>MNRQELITEALKARDMAYAPYSKFQVGAALLTKDGKVYRGCNIENAAYSMCNHAEQTALFKAVSEGDTEFQMLAVAADTPGPVSPCGACRQVISELCTKDVIVVLTNLQGQIKEMTVEELLPGAFSSEDLHDERKL[4x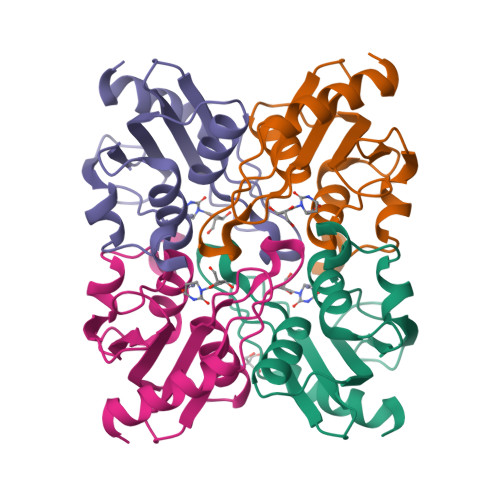]>SMKELSTIQKREKLNTVERIGSEGPGGAYHEYVIKSNS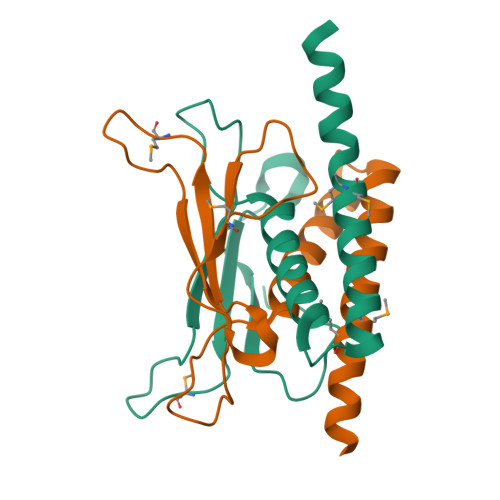MDSQGNYDVYETIKFQKGARKEEKSQHGVIDSDLLEIVRDRLKSFQAGPFSSRENACALTHVEEALMWMNRRVEDRIERNVLGTNTK[5x]>MAEKRTGLAEDGAKSVYERLKNDRAPYETRAQNCAQYTIPSLFPKDSDNASTDYQTPWQAVGARGLNNLASKLMLALFPMQTWMRLTISEYEAKQLLSDPDGLAKVDEGLSMVERIIMNYIESNSYRVTLFEALKQLVVAGNVLLYLPEPEGSNYNPMKLYRLSSYVVQRDAFGNVLQMVTRDQIAFGALPEDIRKAVEGQGGEKKADETIDVYTHIYLDEDSGEYLRYEEVEGMEVQGSDGTYPKEACPYIPIRMVRLDGESYGRSYIEEYLGDLRSLENLQEAIVKMSMISSKVIGLVNPAGITQPRRLTKAQTGDFVTGRPEDISFLQLEKQADFTVAKAVSDAIEARLSFAFMLNSAVQRTGERVTAEEIRYVASELEDTLGGVYSILSQELQLPLV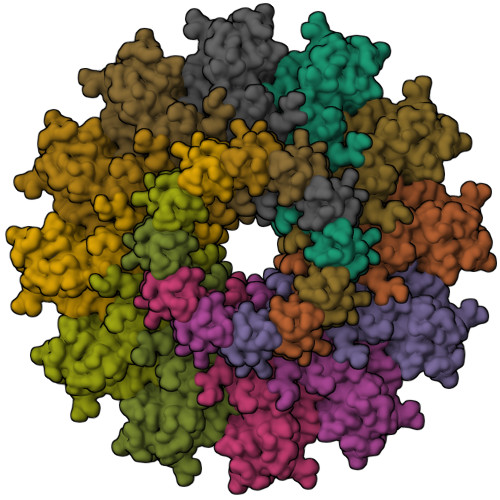RVLLKQLQATQQIPELPKEAVEPTISTGLEAIGRGQDLDKLERCVTAWAALAPMRDDPDINLAMIKLRIANAIGIDTSGILLTEEQKQQKMAQQSMQMGMDNGAAALAQGMAAQATASPEAMAAAADSVGLQPGI[12x]>GASGDVCQDCIQMVTDIQTAVRTNSTFVQALVEHVKEECDRLGPGMADICKNYISQYSEIAIQMMMHMQPKEICALVGFCDE[2x]

Four mature saposins (SapA, SapB, SapC, and SapD) result from proteolysis of the precursor prosaposin as it traffics to the lysosome. The saposin family members are disulfide-linked, four-helix bundles that usually form dimers. SapB presents a variety of ligands to several lysosomal hydrolases, including arylsulfatase A, β-galactosidase (GLB1), and α-galactosidase A (GLA). One cargo, globotriaosylceramide (Gb3), is presented exclusively by SapB to GLA for removal of the terminal α-galactose, and failure of this process leads to accumulation of Gb3 in the lysosome and ultimately results in Fabry disease.

To determine the molecular basis for SapB binding and presenting Gb3, we expressed and purified recombinant human SapB from E. coli and co-crystallized it at lysosomal pH in the presence of Gb3-NBD. Crystals took months to grow and were bright yellow, strongly indicative of NBD from the ligand in the crystal. Third, we dissolved washed crystals in 0.1 % formic acid, subjected the sample to liquid-chromatography mass spectrometry (LC-MS) analysis, which indicated the presence of both SapB and Gb3-NBD. The SapB structure revealed a homodimer consisting of helical V-shaped monomers that form a ~2,900 Å3 binding cavity lined with hydrophobic residues. Given the above evidence for Gb3-NBD in the crystals, we were surprised to see only weak density in the ligand-binding cavity. Additionally, several hydrophobic residues on one face of a helix in the binding cavity showed little density beyond the beta carbon. We interpret the result as a collection of disordered ligands in the hydrophobic cavities of the SapB molecules in the crystalline state. Absent any cargo, the binding cavity collapses, and the cavity volume is minimal; but the presence of two Gb3-NBD increases the pocket volume closer to that seen in the crystal structure, suggesting that the SapB dimer in the crystal structure contains two or more ligands. Moreover, because the chains of the SapB:Gb3-NBD dimer align well with SapB dimers containing ligands, we propose that our structure represents an open and multi-ligand-bound SapB. Our simulations indicate that an open SapB dimer binds at least two Gb3-NBD molecules.> MKNTPQHKLFFVVALLLVVQILAGCKSSSSTTAGSTENSSSSTPDPDTGTTTPDPIEPEVVPPVTPPSVDSNSREVIPLWEDKVADGKAWSTHVYSALDKLGPNLLDVIPADRSLFCPKYSSLSYAQRKQYWAFVLSSMVRFESNFKTAMSYTEDFNDSNGNRVISRGLLQISIESGNAYGCGFKSTKDLHDPLQNLSCGIRILDRWVSRDGRIAGKVDGAWKGGARY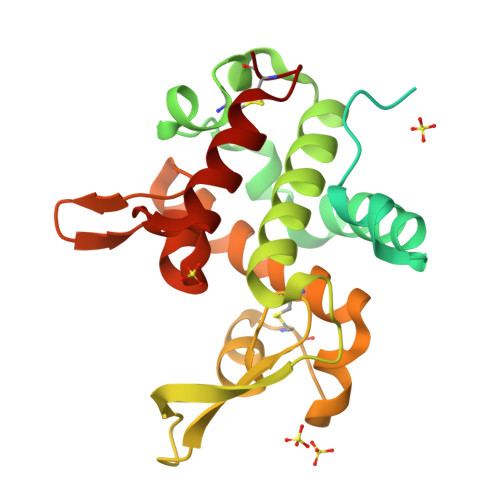WSVLRAGDKTSYKSIVSWSQNLSICK>[2x]GHMDRAPLTATAPQLDDEEMYSAHMPAHLRCDACRAVAYQMWQNLAKAETKLHTSNSGGRRELSELVYTDVLDRSCSRNWQDYGVR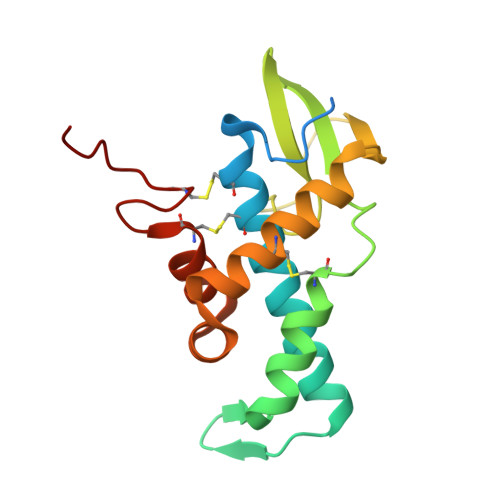EVDQVKRLTGPGLSEGPEPSISVMVTGGPWPTRLSRTCLHYLGEFGEDQIYEAHQQGRGALEALLCGGPQGACSEKVSAT1-(6-hydroxypyridin-3-yl)-4-(methylamino)butan-1-one | 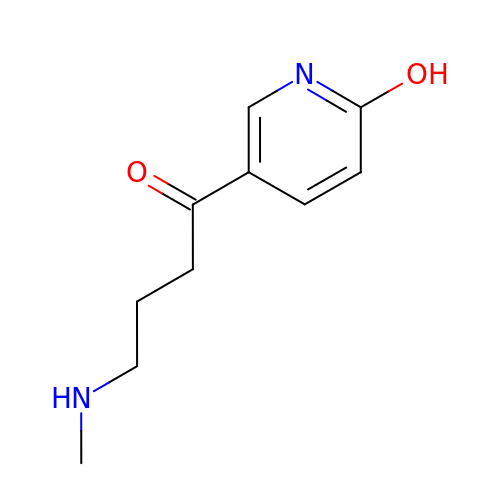C10 H14 N2 O2 | UMLOUOBDBGOHHR-UHFFFAOYSA-N>[12x]MA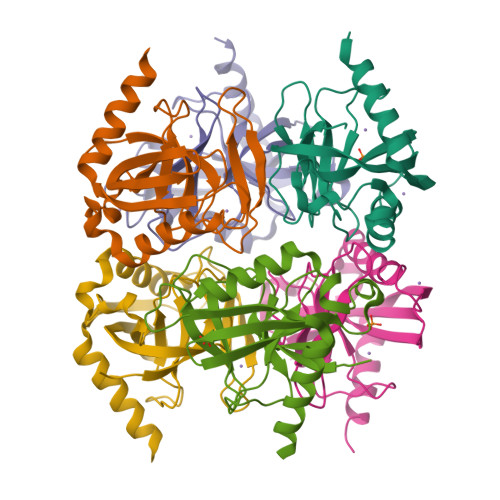HHHHHHAMQFDVTIEIPKGQRNKYEVDHETGRVRLDRYLYTPMAYPTDYGFIEDTLGDDGDPLDALVLLPQPVFPGVLVAARPVGMFRMVDEHGGDDKVLCVPAGDPRWDHVQDIGDVPAFELDAIKHFFVHYKDLEPGKFVKAADWVDRAEAEAEVQRSVERFKAGTH> SHMASMKKKGSVVIVGRINLSGDTAYAQQTRGEEGCQETSQTGRDKNQVEGEVQIVSTATQTFLATSINGVLWTVYHGAGTRTIASPKGPVTQMYTNVDKDLVGWQAPQGSRSL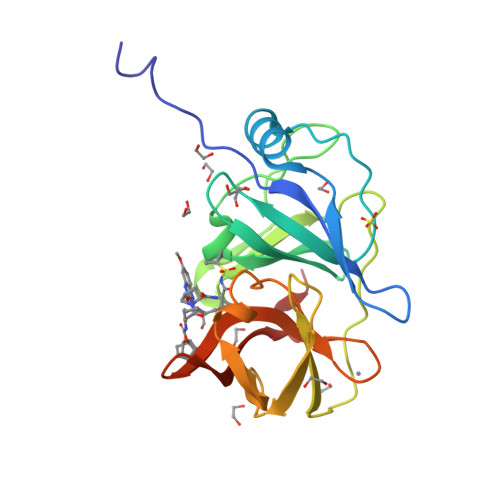TPCTCGSSDLYLVTRHADVIPVRRRGDSRGSLLSPRPISYLKGSSGGPLLCPAGHAVGIFRAAVSTRGVAKAVDFIPVESLETTMRS> MSAILKAPGVYIEEDASLALSVSNSATAVPVFIGKFTPTVVDSIQVCTRISNWLEFTSSFSLAPTVEIVVQSNTESESESETYHYIETINLSPAVEALRLYFQNGGGACYIYPLNDAEDELVLAAIPEVIEQKGDITLLVCPELDLDYKTKIYGAVSSLLNDNKVGYFLIADSNDGESVSGVWNSAKAAAYYPQLETNLKFSTLPGDKDIRISGYQDDDETHKPKNLDELRTINEALAQDIDARLLEEKQRAVIIPPSAAIAGIYCQTDNRRGVWKAPANVALTGIGSLLDKVDDERQGEMNDKGINVIRSFTDRGFMVWGARTCVDAANISWRYIPVRRLFNSVERDIR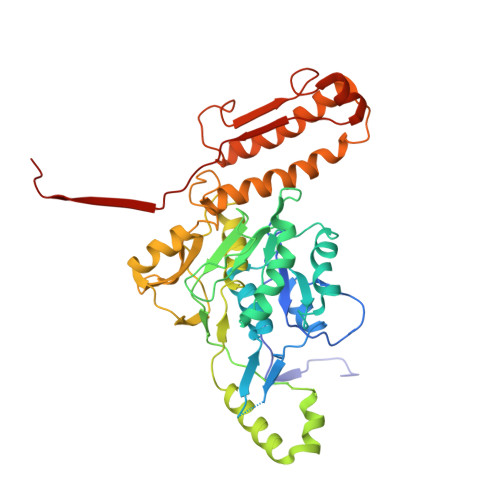QALRAVLFETNSQPTWVRAKAAVDQYLYTLWQKNALMGARPEEAYFVQIGQDITMSEADIKQGKMIMTVGLAAVRPAEFIILQFTQDVVQ>LRTNLTDRQLAEEYLYRYGYTRVAEMRGESKSLGPALLLLQKQLSLPETGELDSATLKAMRTPRCGVPDLGRFQTFEGDLKWHHHNITYWIQNYSEDLPRAVIDDAFARAFALWSAVTPLTFTRVYSRDADIVIQFGVAEHGDGYPFDGKDGLLAHAFPPGPGIQGDAHFDDDELWSLGKGQGYS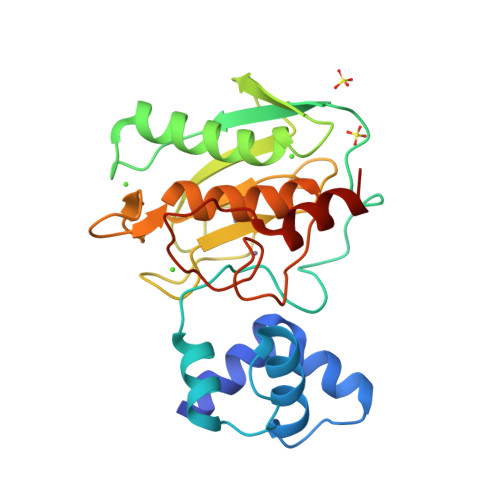LFLVAAHEFGHALGLDHSSVPEALMYPMYRFTEGPPLHKDDVNGIRHLYGP[2x]>[4x]GGHMTRRGKIVCTLGPATQRDDLVRALVEAGMDVARMNFSHGDYDDHKVAYERVRVASDATGRAVGVLADLQGPKIRLGRFASGATHWAEGETVRITVGACEGSHDRVSTTYKRLAQDAVAGDRVLVDDGKVALVVDAVEGDDVVCTVVEGGPVSDNKGISLPGMNVTAPALSEKDIEDLTFALNLGVDMVALSFVRSPADVELVHEVMDRI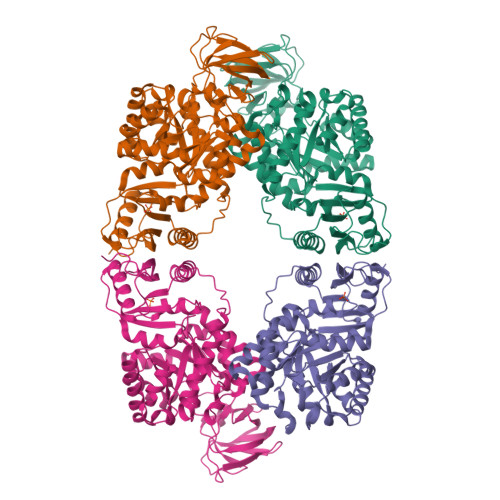GRRVPVIAKLEKPEAIDNLEAIVLAFDAVMVARGDLGVELPLEEVPLVQKRAIQMARENAKPVIVATQMLDSMIENSRPTRAEASDVANAVLDGADALMLSGETSVGKYPLAAVRTMSRIICAVEENSTAAPPLTHIPRTKRGVISYAARDIGERLDAKALVAFTQSGDTVRRLARLHTPLPLLAFTAWPEVRSQLAMTWGTETFIVPKMQSTDGMIRQVDKSLLELARYKRGDLVVIVAGAPPGTVGSTNLIHVHRIGEDDV>MTVNEMREWLRNWVANATGQSADAIDESTPMVELGLSSRDAVAMASDIEDLTGVTLTATVAFRHPTIESLATVIIEGEPEPEPYDEDEDWSRTRDVEDIAIVGVATRFPGDLNTPDEMWEALLEGKDCVTDLPEDRWTEFLDEPRIAERVKKARTRGGYLTDIKGFDSEFFALSKMEADNIDPQQRMALELTWEALEHARIPASSLRGESVGVYIGSSTNDYSFLAMSDPSIAHPYAITGTASSIIANRVSYFYDFRGPSVAVDTACSSSLVATHQGVQALRAGEADVAIVGGVNALVTPLVTVGFDEVGGVLAPDGRIKSFSSDADGYARSEGGGMLVLKRISDARRDGDQILAVIAGSAVNHDGRSNGLLAPNPDAQAEVLRKAYKDAGINPRDVDYIEAHGTGTILGDPIEADALGRIVGKGRPADKPALLGAVKSNLGHLESAAGAASLAKMTLALANDKLPPSINYAGPNPYIDFEKERLKVNDTVSDWPRYSGKAIAGVSGFGFGGANAHVVMREVLAGDLVEPEPEPEPEAKPEKSEADAVYVGGVRMDEYGEFIDEDEPAEGGDAYPSYDEDSYELPGITEAAQRLLEQAREELEAKEAEEPTKQLVPLAVSAFLTSRKRQAAAELADWIDSPEGRASSLESIGRSLSRRNHGRSRAVVLAHDHDEAIKGLRALAEGKQHPSVLSADGPVTNGPVWVLAGFGAQHRKMGKSLYLRNEVFAEWINKVDALIQDERGYSILELILDDNVDYTDATCEYPIEVVQLVIFAIQIALGELLRHHGAKPAAVVGQSLGEAAASYFAGGLSLADATRTICSRSHLMGEGEAMLFGEYIRLMALVEYSADEIKTVFSDYPDLEVCVYAAPTQTVIGGPPDQVDAIIARAESEGKFARKFQTKGASHTQQMDPLLGELAAELQGIEPKPLTTGYFSTVHEGTFIRPGSAPIHDVDYWKKGLRHSVYFTQGIRNAVDNGHTTFLELAPNPVALMQVGLTTASAGLHDAQLIATLARKQDEVESMISAMAQLYVHGHDLDFRTLFPRRSKGLAGALDFANIPPTRFKRKEHWLPAHFTGDSSAVMPGNHVATPDGRHVWEFVPRGKTDLAALVKAAAAQVLPDAKLAAFEQRAVPADNARLVTTLTRHPGGATVQVHARVEESFTLVYDAIVARANGAGVTALPVAVGAGVAVSGDVAGEGAGASVIEDDEPDAEILQDNLTAGAGMGADFQKWDPNSGETIGQRLGTIVGAAMGYEPEDLPWEVPLIELGLDSLMAVRIKNRVEYDFDLPPIQLTAVRDANLYNVEELIRYAIEHRDEVEQIAESQKGKTAEEIAAEQSELLGGASTVAELEAKLAEAGHPLAAKDSEDSENSEDNAAGAAAAAEASAVEGLEIPPPPTDPTGPGGAPIPPPPSDPSGPAQAASATDAPAGTVNKATAAAAAAKVLTQEAVTEALGADVPPRDAAERVT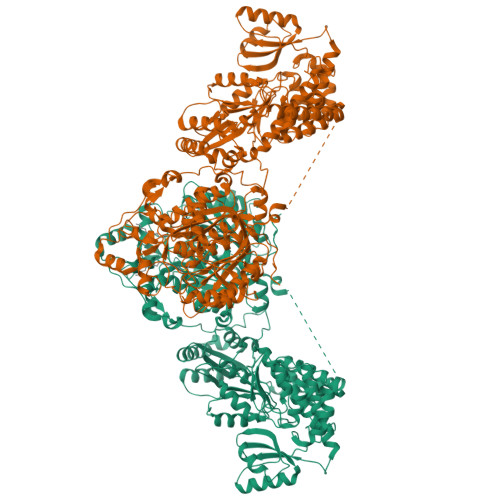FATWAIVTGKSPGGIFNELPTVSEETAKKMAERLSERAEGTITVEDVLGAKTIEGLATIVREQLEEGVVDGFVRTLRPPKEGSNAVPLFVFHPAGGSTVVYEPLMKRLPADVPVYGLERVEGSIEERAAEYVPKLLEMHKGPFVLAGWSLGGALAYACAIGLKQSGADVRFVGLIDTVLPGEPIDQSKEGMRARWDRYARFAERTFNVEIPAIPYEELEKLDDEGQVKYVLEIVKESGVQIPGGIIEHQRTSYLDNRALDTVDIKPYDGHVTLYMADRYHDDAIVFEPAYATRKPDGGWGSFVSDLEVVHIGGEHIQAIDEPYIAKVGAHMSEALNRIEAQASKEDGAK[2x]3-azanylphenazin-2-ol | C12 H9 N3 O | 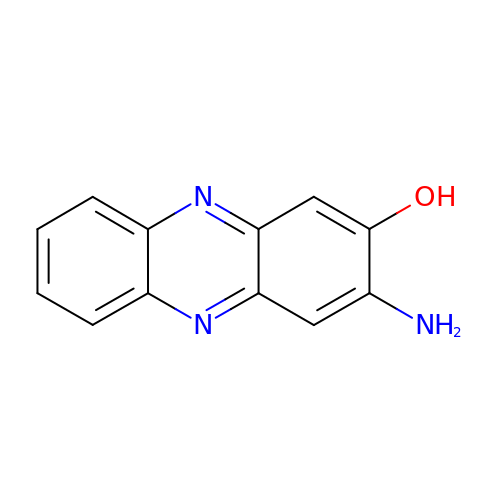AJIRUIWLEVHQMU-UHFFFAOYSA-N> MYKVPKGLEHYQKMFQKEVTVNDLKKYLIGSDKEYRITRRDSYMGDISDPEVILEYGVYPAFIKGYTQLKANIEEALLEMSNSGQALDIYQAVQTLNAENMLLNYYESLPFYLNRQSILANITKALKDAHIREAMAHYKLGEFAHYQDTMLDMVER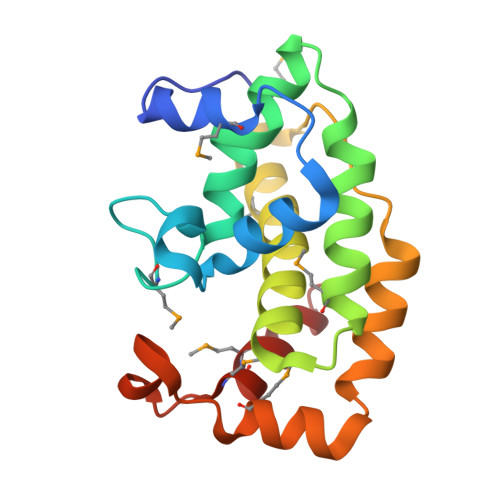TIETF> VKLSEDQEHYIKGVWKDVDHKQITAKAL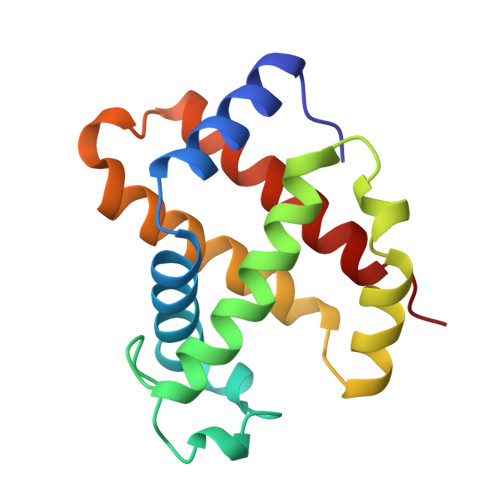ERVFVVYPWTTRLFSKLQGLFSANDIGVQQHADKVQRALGEAIDDLKKVEINFQNLSGKHQEIGVDTQNFKLLGQTFMVELALHYKKTFRPKEHAAAYKFFRLVAEALSSNYH>APITAYAQQTRGLLGCIITSLTGRDKNQVEGEVQIMSTATQTFLATCINGVCWTVYHGAGTRTIASPKGPVIQMYTNVDQDLVGWPAPQGSRSLTPCTCGSSDLYLVTRHADVIPVRRRGDSRGSLLSPRPISYLKGSSGGPLLCPAGHAVGLFRAAVCTRGVAKAVDFIPVENLETTMRS[2x];>KGSVV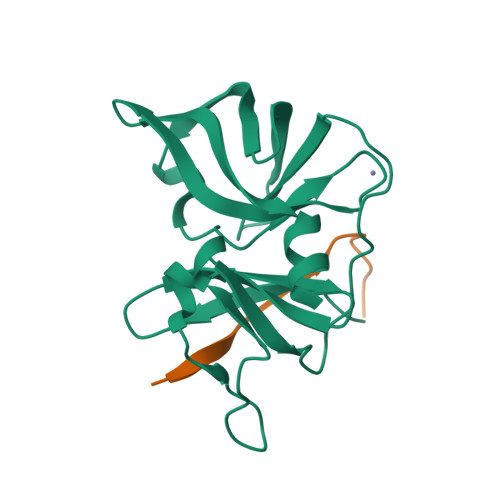IVGRIVLSGKPAIIPA[2x]Deacetylase from the extremophile Pyrococcus chitonophagus has been analyzed by X-ray crystallography, small-angle X-ray scattering, differential scanning calorimetry, isothermal titration calorimetry and NMR to determine its structure, thermodynamics and enzymatic properties. It is a hexameric, zinc-containing metalloenzyme that retains its structural integrity up to temperatures slightly exceeding 100 °C. It removes the acetyl group specifically from the non-reducing end of the sugar substrate. Pch-Dac crystallizes as ‘a dimer of trimers’, with two doughnut-shaped trimers stacked back-to-back along a molecular three-fold axis, with a 8–10 Å channel through the middle of this assembly.

Orthorhombic crystals, Pch-Dac-anom, used for identifying the metal cation, have one hexamer in the asymmetric unit. The presence of Zn2+ in the crystal structure of Pch-Dac was confirmed by X-ray anomalous dispersion. Energy scan performed on the Pch-Dac-anom crystals revealed X-ray absorption profile characteristic of zinc, while anomalous density maps clearly identified the Zn2+ sites as peaks at the level of 18–25 r.m.s.d. In Pch-Dac and Pch-Dac-anom, there was no ligand in the substrate-binding sites and the coordination sphere of Zn2+ consists of the three conserved His-Asp-His residues and a single water molecule that occupies the same position as the carbonyl oxygen of the substrate’s N-acetyl group in the Pch-Dac-lig complex. The same hexameric assembly is observed regardless of crystal packing and probably represents the biologically relevant oligomeric form of the enzyme.

>[6x]MFEEINDFETAFKRLLNEVLEFDLQNPLKDVKKVLCIEPHPDDCVIGMGGTIKRLTDRGIEVIYICMTDGYMGTTDENITGHELAQIRRKEEEESAKMLGVKKIYWLNYRDTELPYSREVRKDLVKIIRKEKPDGVFLPDPWLPYEAHPDHRATGFLALDAVAFSPLPNFSNIDLDIGLKPHSVSFIGLYYTSRPNYFVDITDVMDLKLKAIRAHKSQFPDDIWETWEPFLRTVALYYGQKAGVKYAEGFRIMPGLFYHITPFAELI>PLLIKNGEIITADSRYKADIYAEGETITRIGQNLEAPPGTEVIDATGKYVFPGFIDPHVHIYLPFMATFAKDTHETGSKAALMGGTTTYIEMCCPSRNDDALEGYQLWKSKAEGNSYCDYTFHMAVSKFDEKTEGQLREIVADGISSFKIFLSYKNFFGVDDGEMYQTLRLAKELGVIVTAHCENAELVGRLQQKLLSEGKTGPEWHEPSRPEAVEAEGTARFATFLETTGATGYVVHLSCKPALDAAMAAKARGVPIYIESVIPHFLLDKTYAERGGVEAMKYIMSPPLRDKRNQKVLWDALAQGFIDTVGTDHCPFDTEQKLLGKEAFTAIPNGIPAIEDRVNLLYTYGVSRGRLDIHRFVDAASTKAAKLFGLFPRKGTIAVGSDADLVVYDPQYRGTISVKTQHVNNDYNGFEGFEIDG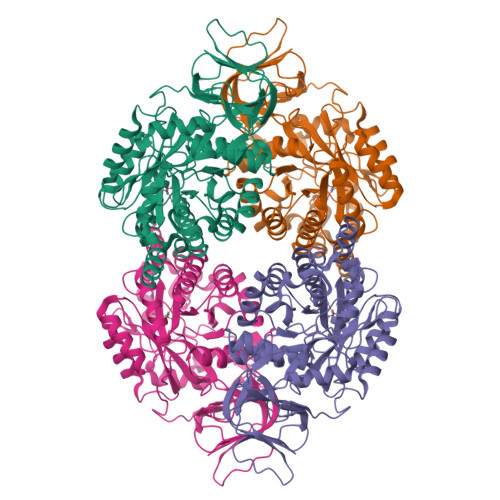RPSVVTVRGKVAVRDGQFVGEKGWGKLLRREPMYF[6x]(2~{R},6~{S})-2,6-dimethyl-4-[6-[5-(1-methylcyclopropyl)oxy-1~{H}-indazol-3-yl]pyrimidin-4-yl]morpholine 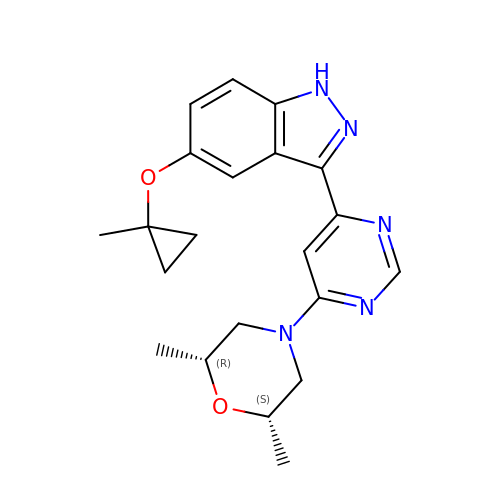| C21 H25 N5 O2 | ATUUNJCZCOMUKD-OKILXGFUSA-N> RVVESDTLINRRYMRATGLGALALLIAACRLIARRLRETRTTLKGSARRF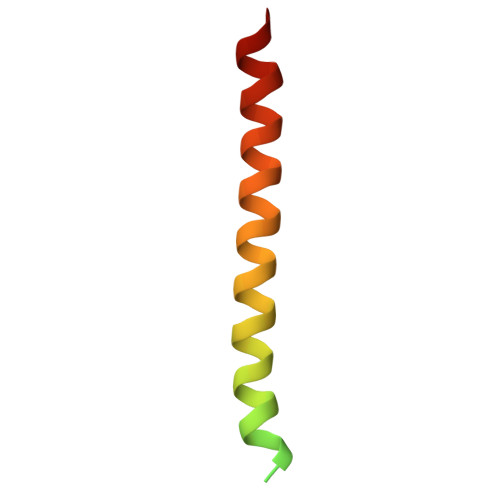NVDLFQVRLILG>[2x]SNASPFDTGPELESQIRNQYGVDVH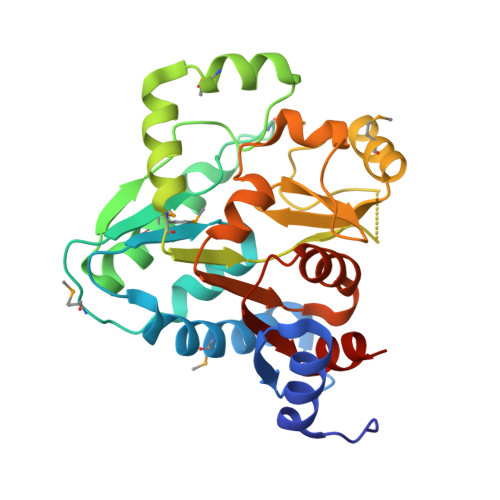VVPVLDTLNEAETLDRVAMQAARTIGPLVDSNAIIGVAWGATLSAVSRHLTRKMTHDSIVVQLNGAGNMQTTGITYASDIMRRFGSAYGARVEQFPVPAFFDHASTKTAMWNERSVQRILDLQARMSIAIFGVGSVDSDYPSHVYAGGYLDEHDLTMLAADDVVGDVATVFFRSDGSSDGITLNERSTGPSHEQLRQVRRRICVVSGASKINGLQGALAAGLATDLILDEASARRLVSFNGH>MSTQYETQGYTINNAGRRLVVDPITRIEGHMRCEVNINDQNVITNAVSCGTMFRGLEIILQGRDPRDAWAFVERICGVCTGVHALASVYAIEDAIGIKVPDNANIIRNIMLATLWCHAHLVHFYQLAGMDWIDVLDALKADPRKTSELAQSLSSWPKSSPGYFFDVQNRLKKFVEGGQLGIFRNGYWGHPQYKLPPEANLMGFAHYLEALDFQREIVKIHAVFGGKNPHPNWIVGGMPCAINIDESGAVGAVNMERLNLVQSIITRTADFINNVMIPDALAIGQFNKPWSEIGTGLSDKCVLSYGAFPDIANDFGEKSLLMPGGAVINGDFNNVLPVDLVDPQQVQEFVDHAWYRYPNDQVGRHPFDGITDPWYNPGDVKGSDTNIQQLNEQERYSWIKAPRWRGNAMEVGPLARTLIAYHKGDAATVESVDRMMSALNLP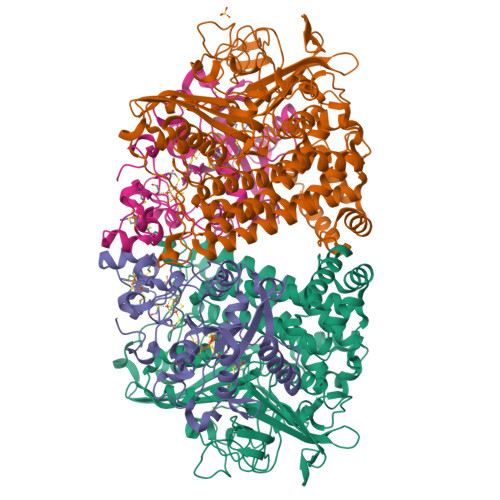LSGIQSTLGRILCRAHEAQWAAGKLQYFFDKLMTNLKNGNLATASTEKWEPATWPTECRGVGFTEAPRGALGHWAAIRDGKIDLYQCVVPTTWNASPRDPKGQIGAYEAALMNTKMAIPEQPLEILRTLHSFDPCLACSTH[2x];>LENKPRIPVVWIHGLECTCCTESFIRSAHPLAKDVILSLISLDYDDTLMAAAGTQAEEVFEDIITQYNGKYILAVEGNPPLGEQGMFCISSGRPFIEKLKRAAAGASAIIAWGTCASWGCVQAARPNPTQATPIDKVITDKPIIKVPGCPPIPDVMSAIITYMVTFDRLPDVDRMGRPLMFYGQRIHDKCYRRAHFDAGEFVQSWDDDAARKGYCLYKMGCKGPTTYNACSSTRWNDGVSFPIQSGHGCLGCAENGFWDRGSFYSRVVDIPQMGTHSTADTVGLTALGVVAAAVGVHAVASAVDQRRRHNQQPTETEHQPGNEDKQARSHHHHHH[2x]>[2x]GHMSITENTSWNKEFSAEAVNGVFVLCKSSSKSCATNDLARASKEYLPASTFKIPSAIIGLETGVIKNEHQVFKWDGKPRAMKQWERDLTLRGAIQV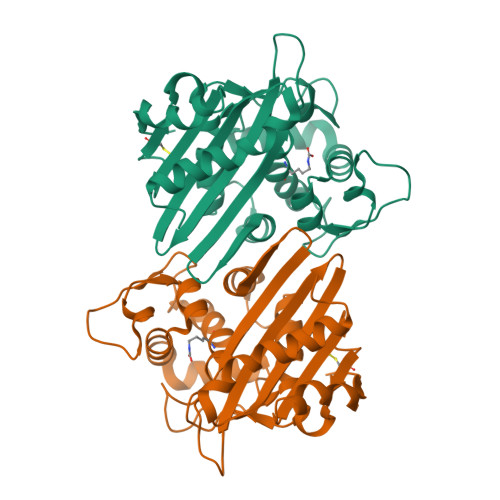SAVPVFQQIAREVGEVRMQKYLKKFSYGNQNISGGIDKFWLEGQLRISAVNQVEFLESLYLNKLSASKENQLIVKEALVTEAAPEYLVHSKTGFSGVGTESNPGVAWWVGWVEKETEVYFFAFNMDIDNESKLPLRKSIPTKIMESEGIIG(2~{S})-2,6-bis(azanyl)-~{N}-oxidanyl-hexanamide 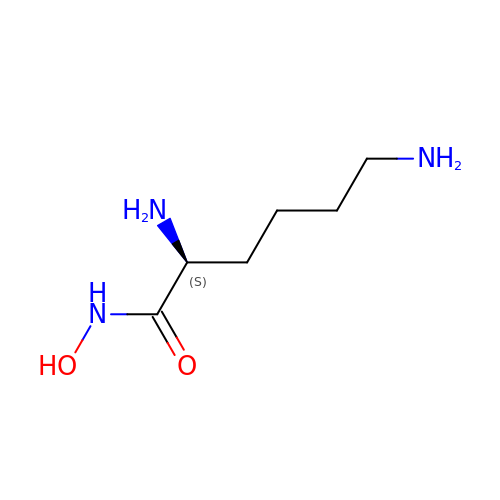| C6 H15 N3 O2 | NZWPVDFOIUKVSJ-YFKPBYRVSA-N>[18x]MVRKVFNDGDILYAEDVNIIGQPFVDGQDLLGHGLKVDDNSLSDEPQNIKTRFYAWYNRFRVTVQSGLTLSVTQGSISVSGNIISFPPQTINAIDNANSFVWIGKTDADPAIALRVSQTLPNVCIPLARVIAASGSVTSVTDLRDVSVDILPPSIPDAVPVGSTIISLIPPTAPIPAGYLELLNSSQNVSRTTYSALFVLWGTYYGNGDGSTTFGVPGTGGRFLRLGGSGLSVGDIGGSNQITIPTNALPSHQHGIPANTHTHSVNDGGHGHTINQTPHSHSISDPGHAHGVPFGAAVDNGNNAFDTGGSPYNNGIGTTQNQTGISVNTANANLSINTSSTGISIQSASTGLTVTSNAGNGQAFQHDQPYLVFRVFVKV;>MTNIVGRIGFLTTGKLGIKLRGVLIDESTTPNTTYLPGIESFFNITANVLTSVSYPETETQNVTATFSIYSVDGSSNPVFPALLSFDAIVPNVASVEFDVLAPTGVVNNQLDTSALRIAKIIANDPALAQKVAGAPYPRGAYSATETYLYGEMVSYFGKNYISKSLSPIINILPTVTDSWYELVITLPESVSVIATGSDTAYGTGWNGSLLVPTQNAVYDKIVTVDAAIATANTNITNLGTAKADLSYVNTQLSADQVVLDALSSGKADLSYVNTQLNSKANLNGAVLVNATTATPPISDNDTSLATTQHVRSFNHSRLAFNAFRGGQQGVPSLSYVTTTAQFNSSSVRSGWGDNFSSNRWLVGEGGTYLITVTTRFATVGGTPPTYFDALLFVGLSGSGVENFLTRSQSVYPSFGYTLSWVGILTFNTGQNVFLNYQVNAVGGGSYSVVLEDVRFSGIQLG[18x]

A-1(L) is a Myoviridae cyanophage isolated in 1970s9 that specifically infects the model cyanobacterium Anabaena sp. PCC 7120. Using cryo-electron microscopy (cryo-EM), we solved the structure of A-1(L) tail machine, which consists of three parts: a 205-Å-long neck, a 1045-Å-long contractile tail with a complicated baseplate, and six pairs of tail fibers. The dodecameric gp2 portal, the pentadecameric gp5 and the hexameric gp7 sequentially constitute the neck of A-1(L), to which five neck fibers are attached. The long and contractile tail of A-1(L) contains 24 rings of gp10 hexamers that form the tube, surrounded by the sheath of 24 helically stacked gp9 hexamers.

A-1(L) possesses two types of tail fibers: six LTFs/gp34 trimers (274 Å long) and six STFs/gp33 trimers (258 Å long), all of which anchor to the baseplate in an upward conformation. Each LTF subunit contains a shoulder and an arm domain, whereas each STF subunit consists of four domains: β-ring, joint, stem and cell wall binding domain (CBD). The shoulder domain (residues Met1-Ile155) of LTF is anchored to the wedge of baseplate, via interacting with the insertion domain (residues Glu81-Gly180) of gp31B and the C-terminal loop (residues Val129-Glu151) of gp32. In contrast, the 180-Å-long arm domain (residues Pro156-Val379) of LTF is folded back and lies along the groove on the sheath. Eighteen β-ring domains (residues Thr2-Gln110) of six trimeric STFs form a ring structure that encircles the distal plane of six wedges, whereas the joint domains (residues Leu111-Gln215) bind to the periphery of six wedges, making the STFs tightly anchor to the baseplate. Moreover, the long helical bundle formed by the stem domains (residues Asn216-Asn282) of STF trimer runs along the groove formed by the trimeric shoulder domain (residues Met1-Ile155) of the LTF. The overall folded conformation of these two types of tail fibers suggested a state of A-1(L) in prior of attachment to the surface of host cell. Structural analysis showed that the arm domain of LTF and the CBD domain of STF most likely possess the binding motifs that recognize the host receptors. Further competition binding assays showed that the arm domain of LTF and the stem-CBD domain of STF could simultaneously bind to the surface of host cells. Altogether, it suggested that the STF/gp33 and LTF/gp34 are indeed RBPs, which recognize and bind to different receptors on the host cell surface.>[2x]MKRAVITGLGIVSSIGNNQQEVLASLREGRSGITFSQELKDSGMRSHVWGNVKLDTTGLIDRKVVRFMSDASIYAFLSMEQAIADAGLSPEAYQNNPRVGLIAGSGGGSPRFQVFGADAMRGPRGLKAVGPYVVTKAMASGVSACLATPFKIHGVNYSISSACATSAHCIGNAVEQIQLGKQDIVFAGGGEELCWEMACEFDAMGALSTKYNDTPEKASRTYDAHRD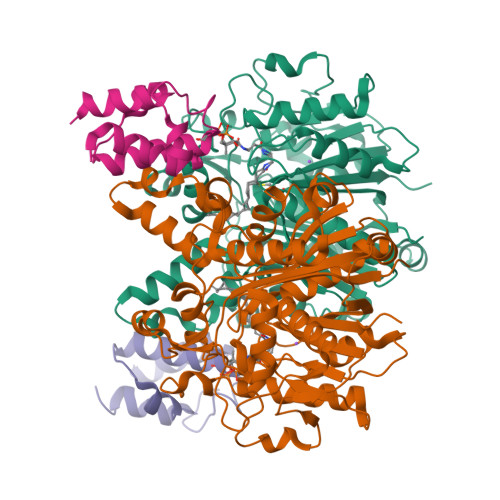GFVIAGGGGMVVVEELEHALARGAHIYAEIVGYGATSDGADMVAPSGEGAVRCMKMAMHGVDTPIDYLNSHGTSTPVGDVKELAAIREVFGDKSPAISATKAMTGHSLGAAGVQEAIYSLLMLEHGFIAPSINIEELDEQAAGLNIVTETTDRELTTVMSNSFGFGGTNATLVMRKLK;>MSTIEERVKKIIGEQLGVKQEEVTNNASFVEDLGADSLDTVELVMALEEEFDTEIPDEEAEKITTVQAAIDYINGHQA[2x]>[2x]MSLNSTQMNKQVIDKYTQRHELYLEQLLNEIIIPAPQIRSALHYALFSGGKRIRPILVYLAGDLIDVDQGVLDIIAAALELTHCYSLIHDDLPAMDNDDLRRGKPSCHKAFDEATAILVGDGMQALAIEVLLMRLSPLL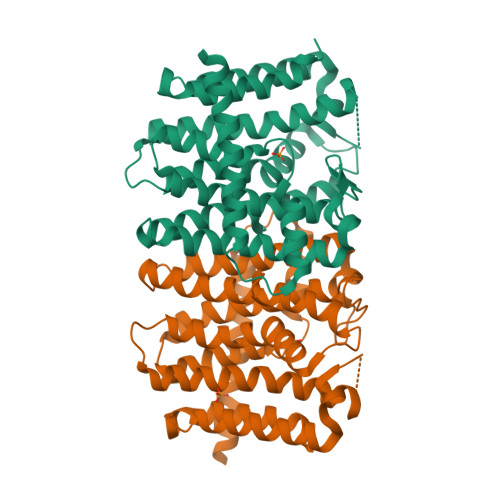PAAQVVAITQVLVNASGISGMVSGQSLDLSELAKSSVTEEQLREIHLLKTGKLILACFEMVLAAQHEVSEQIKSALRTYGKHIGLVFQMQDDYLDLYAPTQILGKGRSSDQANQKTTFATLFNKQQLEEEIAVHYQIAMDSLRLFGSKAAALIELTKQLQNRSNLSEGHHHHHH>[5x]SQLHYTVQEEQEHGTFVGNIAEDLGLDITKLSARGFQTVPNSRTPYLDLNLETGVLYVNEKIDREQICKQSPSCVLHLEVFLENPLELFQVEIEVLDINDNPPSFPEPDLTVEISESATPGTR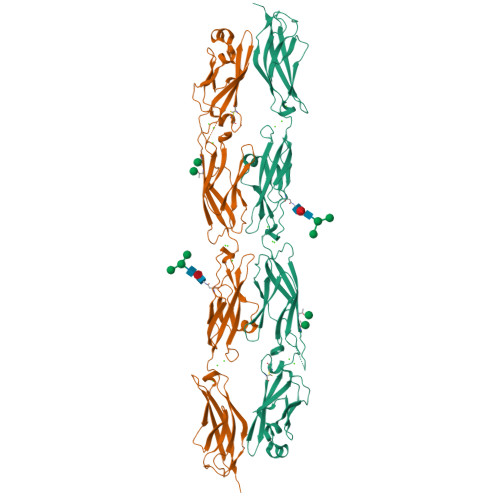FPLESAFDPDVGTNSLRDYEITPNSYFSLDVQTQGDGNRFAELVLEKPLDREQQAVHRYVLTAVDGGGGGGVGEGGGGGGGAGLPPQQQRTGTALLTIRVLDSNDNVPAFDQPVYTVSLPENSPPGTLVIQLNATDPDEGQNGEVVYSFSSHISPRARELFGLSPRTGRLEVSGELDYEESPVYQVYVQAKDLGPNAVPAHCKVLVRVLDANDNAPEISFSTVKEAVSEGAAPGTVVALFSVTDRDSEENGQVQCELLGDVPFRLKSSFKNYYTIVTEAPLDREAGDSYTLTVVARDRGEPALSTSKSIQVQVSDHHHHHH> MHHHHHHENLYFQGAASMNKKTKLIHGGHTTDDYTGAVTTPIYQTSTYLQDDIGDLRQGYEYSRTANPTRSSVESVIAALENGKHGFAFSSGVAAISAVVMLLDKGDHIILNSDVYGGTYRALTKVFTRFGIEVDFVDTTHTDSIVQAIRPTTKMLFIETPSNPLLRVTDIKKSAEIAKEHGLISVVDNTFMTPYYQNPLDLGIDIVLHSATKYLGGHSDVVAGLVATSDDKLAERLAFISNSTGGILGPQDSYLLVRGIKTLGLRM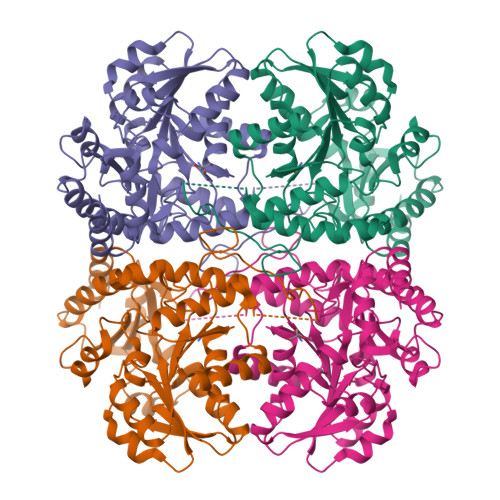EQINRSVIEIIKMLQAHPAVQQVFHPSIESHLNHDVHMAQADGHTGVIAFEVKNTESAKQLIKATSYYTLAESLGAVESLISVPALMTHASIPADIRAKEGITDGLVRISVGIEDTEDLVDDLKQALDTL> EQSSSEIKIVRDEYGMPHIYANDTWHLFYGYGYVVAQDRLFQMEMARRSTQGTVAEVLGKDFVKFDKDIRRNYWPDAIRAQIAALSPEDMSILQGYADGMNAWIDKVNTNPETLLPKQFNTFGFTPKRWEPFDVAMIFVGTMANRFSDSTSEIDNLALLTALKDKYGVSQGMAVFNQLKWLVNPSAPTTIAVQESNYPLKFNQQNSQTAALLPRYDLPAPMLDRPAKGADGALLALAAGKNRETIAAQFAQGGANGLAGY;> SNMWVIGKSKAQDAKAIMVNGPQFGWYAPAYTYGIGLHGAGYDVTGNTPFAYPGLVFGHNGVISWGSTAGFGDDVDIFAERLSAEKPGYYLHNGKWVKMLSREETITVKNGQAETFTVWRTVHGNILQTDQTTQTAYAKSRAWDGKEVASLLAWTHQMKAKNWQEWTQQAAKQALTINWYYADVNGNIGYVHTGAYPDRQSGHDPRLPVPGTGKWDWKGLLPFEMNPKVYNPQSGYIANWANSPQKDYPASDLFAFLWGGADRVTEIDRLLEQKPRLTADQAWDVIRQTSRQDLNLRLFLPTLQAATSGLTQSDPRRQLVETLTRWDGINLLNDDGKTWQQPGSAILNVWLTSMLKRTVVAAVPMPFDKWYSASGYETTQDGPTGSLNISVGAKILYEAVQG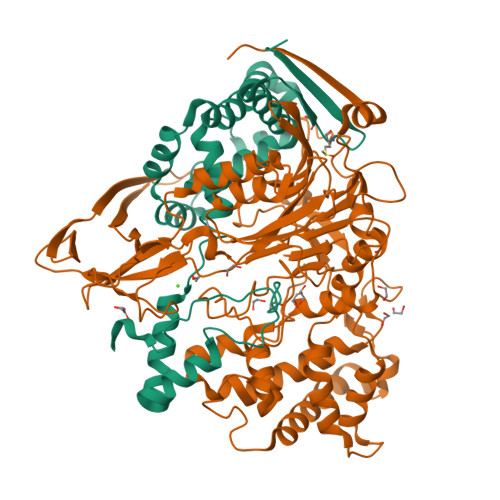DKSPIPQAVDLFAGKPQQEVVLAALEDTWETLSKRYGNNVSNWKTPAMALTFRANNFFGVPQAAAEETRHQAEYQNRGTENDMIVFSPTTSDRPVLAWDVVAPGQSGFIAPDGTVDKHYEDQLKMYENFGRKSLWLTKQDVEAHKESQEVLHVQR>[4x]MNHKVHHHHHHIEGRHMPFEIVFDGAKEFADLIATASNLIDEAAFKITEEGVSMRAMDPSRVVLIDLNLP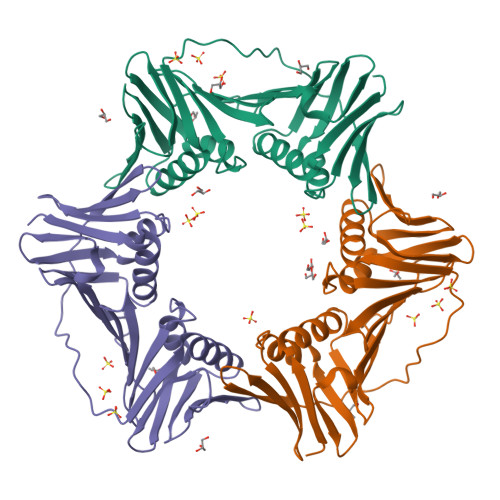ESIFSKYEVEEPETIGINMDHFKKILKRGKSKDTLILRKGDENFLEITFEGTAKRTFRLPLIDVEELELELPELPFTAKVVLLGEVLKEAIKDASLVSDSLKFIAKEDEFTMKAEGETNEVEIKLTLEDEGLLDLEVEEETRSAYGISYLADMVKGIGKADEVTLRFGTEMPLQMDYFIRDEGKLTFLLAPRVEE Human Artemis, 692 residues in length, contains an N-terminal catalytic domain (∼370 residues) with nuclease activity and a C-terminal regulatory region for DNA-PKcs interaction. Based on amino acid sequence analysis, the N-terminal Artemis catalytic domain has been classified in the β-CASP (CPSF, Artemis, SNM1, and Pso) family with a β-CASP domain fused to a conserved metallo-β-lactamase fold. We found that Artemis displays an overall fold similar to that of other members of the SNM1 family and CPSF-73 but also shows unique features, such as a novel zinc binding site in the β-CASP domain and a distinct substrate binding surface. Artemis is able to process several different DNA substrate structures, such as blunt ends, hairpin ends, 5′ overhangs, 3′ overhangs, and symmetrical bubble DNA structures.

Crystal form 2 was obtained when a hairpin DNA was used. Crystals of both forms were dark blue, indicating that the different DNA ligands, each with a Cyanine5 dye tag, were present in the crystals. However, after the structures were solved, the DNA could not be built into the structures of either crystal form, which resulted in a higher Rwork/Rfree gap during refinement. Some broken stacking electron density was observed around the 2-fold axis of crystal form 1 and a solvent channel in crystal form 2. The unsolved electron density in crystal form 2 was not in close proximity to the active site identified by the metal center. This indicated that the DNA was present in the solvent channel but bound promiscuously. Crystal form 2 contained two Artemis molecules in the asymmetric unit and, for both molecules, residues 3–361, except residues 54, 299, and 300, were refined in the final structures. The three copies of Artemis were very similar to each other, with a root mean square deviation (r.m.s.d.) in the range of 0.37 to 0.60 Å. The restructuring of this loop and the coordination of Cys-256 induced a ∼40° rotation of helix αF from its position in SNM1A and SNM1B. The same position of helix αF was also observed for the structures from crystal form 2.

>SSFEGQMAEYPTISIDRFDRENLRARAYFLSHCHKDHMKGLRAPTLKRRLECSLKVYLYCSPVTKELLLTSPKYRFWKKRIISIEIETPTQISLVDEASGEKEEIVVTLLPAGHCPGSVMFLFQGNNGTVLYTGDFRLAQGEAARMELLHSGGRVKDIQSVYLDTTFCDPRFYQIPSREECLSGVLELVRSWITRSPYHVVWLNCKAAYGYEYLFTNLSEELGVQVHVNKLDMFRNMPEILHHLTTDRNTQIHACRHPKAEEYFQWSKLPCGITSRNRIPLHIISIKPSTMWFGERSRKTNVIVRTGESSYRACFSFHSSYSEIKDFLSYLCPVNAYPNVIPVGTTMDKVVEILKPLCRSSQSTEPKKGENLYFQ[2x]>[4x]GPGSEFPGVEPGHFGVCVDSLTSDKASVPIVLEKLLEHVEMHGLYT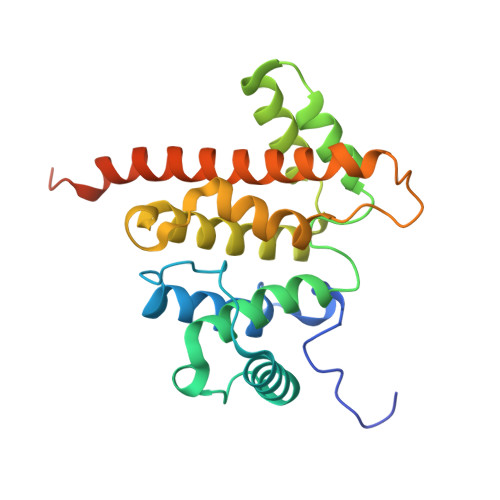EGLYRKSGAANRTRELRQALQTDPAAVKLENFPIHAITGVLKQWLRELPEPLMTFAQYGDFLRAVELPEKQEQLAAIYAVLEHLPEANHNSLERLIFHLVKVALLEDVNRMSPGALAIIFAPCLLRCPDNSDPLTSMKDVLKITTCVEMLIKEQMRKYKVKMEEISQLEAAESIAFRRLSLLRQNA> XXXXXXXXXXXXXXXXXXMATRQRLMRGIAGLLHQQGQQSSCSQLLMTSAAAASASASSVATGPSHQPALLLRAGSALRGVTTSAPTFNGSLSSLLREEVDYERKNYERPAQISGGPPAPFKLTEAPGDTLLTLTRTFGAEEINVDLHVNSQPSPEYDGEDGDEGISVVAFNVSVAKGDRVLLFECESDGNSVN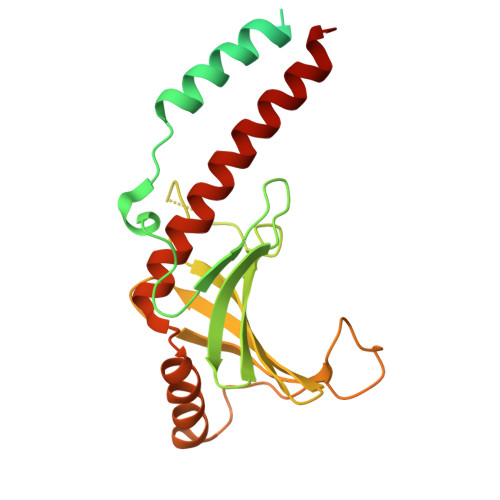INHVSLEPKEGLGSESMYSGPVFDELDDNLQGQFGKYLEDRGITAELGEYLRFLIYDKEQREYQNWLSEVEAFVGGK>MASWSHPQFEKGADDDDKVPDPTSVDSVKYSKIKGIPKLDDANDAGGKHSLECTLILTEGDSAKSLAVSGLGVIGRDRYGVFPLRGKILNVREASHKQIMENAEINNIIKIVGLQYKKSYDDAESLKTLRYGKIMIMTDQDQDGSHIKGLLINFIHHNWPSLLKHGFLEEFITPIVKASKNKQELSFYSIPEFDEWKKHIENQKAWKIKYYKGLGTSTAKEAKEYFADMERHRILFRYAGPEDDAAITLAFSKKKIDDRKEWLTNFMEDRRQRRLHGLPEQFLYGTATKHLTYNDFI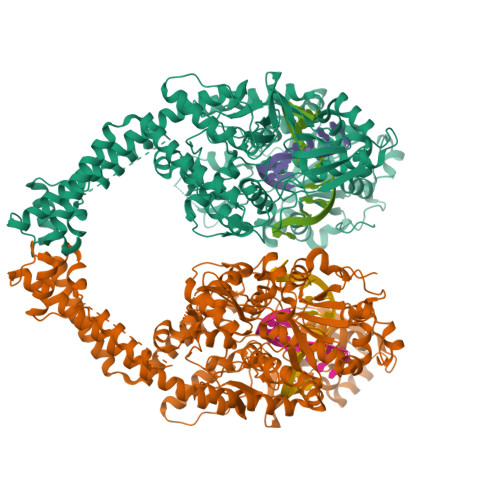NKELILFSNSDNERSIPSLVDGFKPGQRKVLFTCFKRNDKREVKVAQLAGSVAEMSAYHHGEQALMMTIVNLAQNFVGSNNINLLQPIGQFGTRLHGGKDAASPRYIFTMLSTLARLLFPAVDDNLLKFLYDDNQRVEPEWYIPIIPMVLINGAEGIGTGWACKLPNYDAREIVNNVRRMLDGLDPHPMLPNYKNFKGTIQELGQNQYAVSGEIFVVDRNTVEITELPVRTWTQVYKEQVLEPMLNGTDKTPALISDYKEYHTDTTVKFVVKMTEEKLAQAEAAGLHKVFKLQTTLTCNSMVLFDHMGCLKKYETVQDILKEFFDLRLSYYGLRKEWLVGMLGAESTKLNNQARFILEKIQGKITIENRSKKDLIQMLVQRGYESDPVKAWKEAQEKAAEEDETQNQHDDSSSDSGTPSGPDFNYILNMSLWSLTKEKVEELIKQRDAKGREVNDLKRKSPSDLWKEDLAAFVEELDKVESQEREDGAPGFSSISAHHHHHHHHHH[2x]>[2x]MRKHPQTATKHLFVSGGVASSLGKGLTASSLGQLLTARGLHVTMQKLDPYLNVDPGTMNPFQHGEVFVTEDGAETDLDVGHYERFLDRNLPGSANVTTGQVYSTVIAKERRGEYLGDTVQVIPHITDEIKRRILAMAQPDADGNRPDVVITEIGGTVGDIESQPFLEAARQVRHYLGREDVFFLHVSLVPYLAPSGELKTKPTQHSVAALRSIGITPDALILRCDRDVPEALKNKIALMCDVDIDGVISTPDAPSIYDIPKVLHREELDAFVVRRLNLPFRDVDWTEWDDLLRRVHEPHETVRIALVGKYVELSDAYLSVAEALRAGGFKHRAKVEICWVASDGCETTSGAAAALGDVHGVLIPGGFGIRGIEGKIGAIAYARARGLPVLGLCLGLQCIVIEAARSVGLTNANSAEFDPDTPDPVIATMPDQEEIVAGEADLGGTMRLGSYPAVLEPDSVVAQAYQTT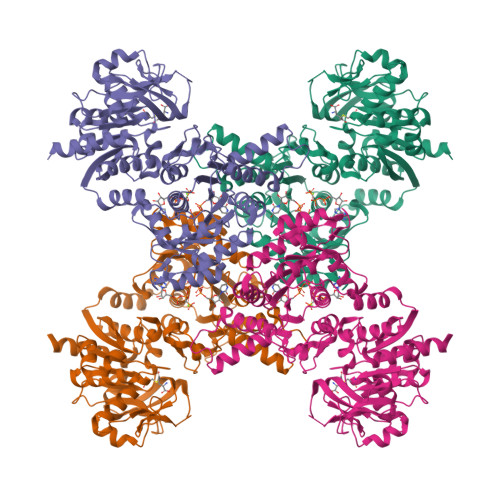QVSERHRHRYEVNNAYRDKIAESGLRFSGTSPDGHLVEFVEYPPDRHPFVVGTQAHPELKSRPTRPHPLFVAFVGAAIDYKAGELLPVEIPEIPEHTPNGSSHRDGVGQPLPEPASRG>MDVVRASRNAKVKGKFRESYLSPAQSVKPKINTEEKLPREKLNPPTPSIYLESKRDAFSPVLLQFCTDPRNPITVIRGLAGSLRLNLGLFSTKTLVEASGEHTVEVRTQVQQPSDENWDLTGTRQIWPCESSRSHTTIAKYAQYQASSFQESLQEEKESEDEESEEPDSTTGTPPSSAPDPKNHHIIKFGTNIDLSDAKRWKPQLQELLKLPAFMRVTSTGNMLSHVGHTILGMNTVQLYMKVPGSRTPGHQENNNFCSVNINIGPGDCEWFAVHEHYWETISAFCDRHGVDYLTGSWWPILDDLYASNIPVYRFVQRPGDLVWINAGTVHWVQATGWCNNIAWNVGPLTAYQYQLALERYEWNEVKNVKSIVPMIHVSWNVARTVKISDPDLFKMIKFCLLQSMKHCQVQRESLVRAGKKIAYQGRVKDEPAYYCNECDVEVFNILFVTSENGSRNTYLVHCEGCARRRSAGLQGVVVLEQYRTEELA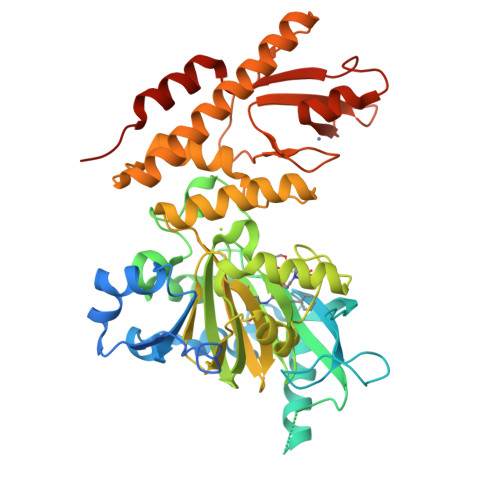QAYDAFTLAPASTSRHHHHHH[2x]> MKDNSTSAVSSWLGYKIQEYRLTQRLLEANNSSCIGFEILDDLEEHTGSTSTFEQDKISTTGRNIVSNHSKDLWKTLSNWMDLIDSGEIDVDNTIFLLFTNKRCHSEVLQLLSTSQATEEASKAFDEILKIVSHPSPSIANYLNNFSKSKTDACRLISKFTYIYGSGSAPHDLRESYKLHRLGALEEHLDEIMYEILGWVSDVLTLAAEKRQPTIV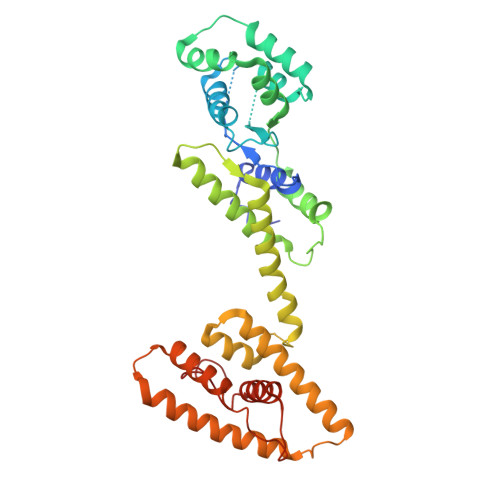RAKDFGARLGEIESKYRQKTILNYFCNRSSESEDVQNTIKDAPNYIKQLNLINVDDSELEEAAIANLETKDAVVEWTLNGDVQDYSYRYYQRELRRCWGIQKQKIHLDFNGRPETEVGQRLYIECLNNVTRYYLENKKVGDFFAHGTLHSMADKLTIGWHPEFDKKLGDPDA> MDETGKELVLVLYDYQEKSPRELTVKKGDILTLLNSTNKDWWKIEVNGRQGFV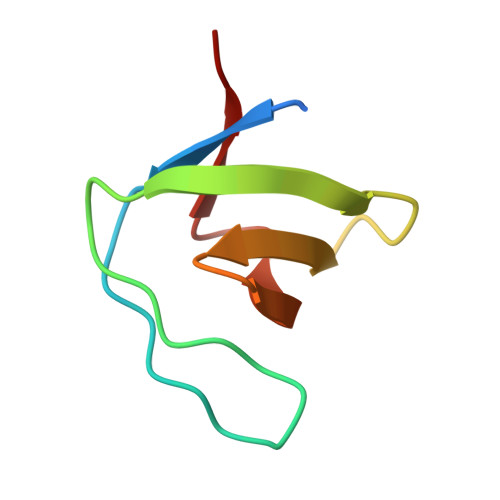PAAYLKKLD>[2x]MSFSRRPKVTKSDIVDQIALNIKNNNLKLEKKYIRLVI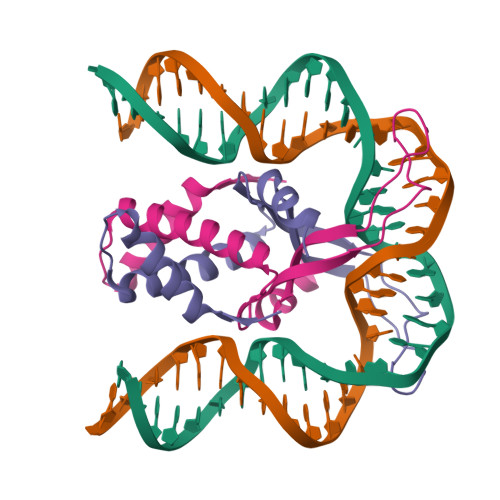DAFFEELKSNLCSNNVIEFRSFGTFEVRKRKGRLNARNPQTGEYVKVLDHHVAYFRPGKDLKERVWGIKG> ERHKILHRL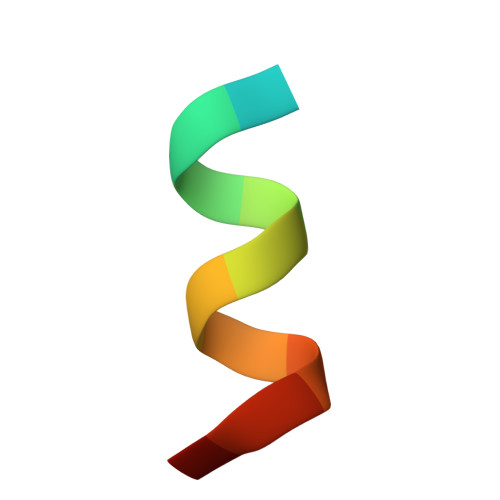LQEG>GHHHHHHHHHHSSGHIEGRHMKPSFSPRNYKALSEVQGWKQRMAAKELARQNMDLGFKLLKKLAFYNPGRNIFLSPLSISTAFSMLCLGAQDSTLDEIKQGFNFRKMPEKDLHEGFHYIIHELTQKTQDLKLSIGNTLFIDQRLQPQRKFLEDAKNFYSAETILTNFQNLEMAQKQINDFISQKTHGKINNLIENIDPGTVMLLANYIFFRARWKHEFDPNVTKEEDFFLEKNSSVKVPMMFRSGIYQVGYDDKLSCTILEIPYQKNITAIFILPDEGKLKHLEKGLQVDTFSRWKTLLSRRVVDVSVPRLHMTGTFDLKKTLSYIGVSKIFEEHGDLTKIAPHRSLKVGEAVHKAELKMDERGTEGA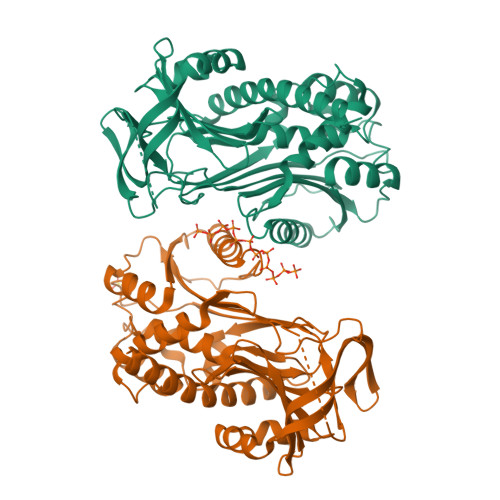AGTGAQTLPMETPLVVKIDKPYLLLIYSEKIPSVLFLGKIVNPIGK[2x]> GPLGSPEFMEPLKVEKFATANRGNGLRAVTPLRPGELLFRSDPLAYTVCKGSRGVVCDRCLLGKEKLMRCSQCRVAKYCSAKCQKKAWPDHKRECKCLKSCKPRYPPDSVRLLGRVVFKLMDGAPSESEKLYSFYDLESNINKLTEDRKEGLRQLVMTFQHFMREEIQDASQLPPAFDLFEAFAKVICNSFTICNAEMQEVGVGLYPSISLLNHSCDPNCSIVFNGPHLLLRAVRDIEVGEELTICYLDMLMTSEERRKQLRDQYCFECDCFRCQTQDKDADMLTGDEQVWKEVQESLKKIEELKAHWKWEQVLAMCQAIISSNSERLPDINIYQLKVLDCAMDACINLGLLEEALFYGTRTMEPYRIFFPGSHPVRGVQVMKVGKLQLHQ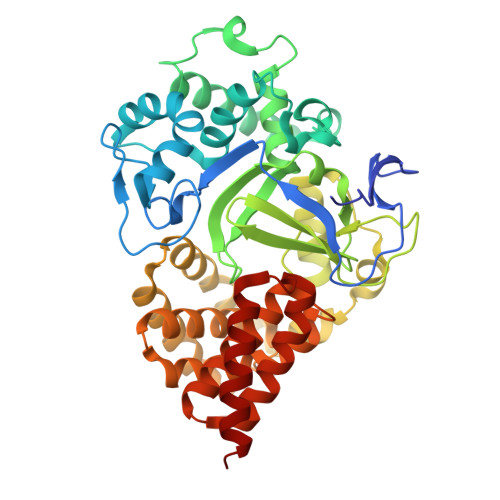GMFPQAMKNLRLAFDIMRVTHGREHSLIEDLILLLEECDANIRAS>[7x]TNTLPHVAFYISVNRAISDEECTFNNSWLWKNEKGSRPFCKDANISLIYRVNLERSLQYGIVGSAAPDAKIVRISLDDDSTGAGIHLNDQLGYRQFGAS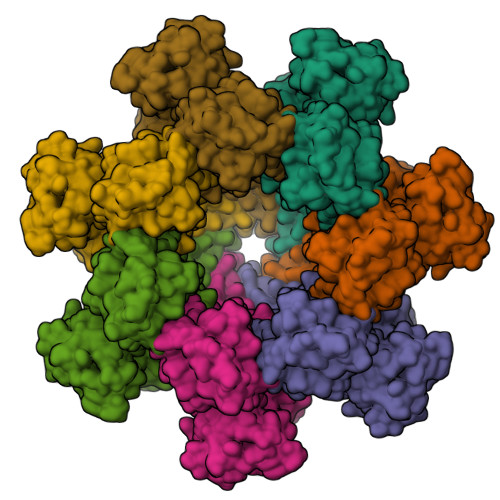YTTLDAYFREWSTDAIAQDYRFVFNASNNKAQILKTFPVDNINEKFERKEVSGFALGVTGGVEVSGDGPKAKLEARASYTQSRWLTYNTQDYRIERNAKNAQAVSFTWNRQQYATAESLLNRSTDALWVNTYPVDVNRISPLSYASFVPKMDVIYKASATETGSTDFIIDSSVNIRPIYNGAYKHYYVVGAHQFYHGFEDTPRRRITKSASFTVDWDHPVFTGGRPVNLQLASFNNRCIQVDAQGRLAANTCDSQQSAQSFIYDQLGRYVSASNTKLCLDGEALDALQPCNQNLTQRWEWRKGTDELTNVYSGESLGHDKQTGELGLYASSNDAVSLRTITAYTDVFNAQESSPILGYTQGKMNQQRVGQDHRLYVRAGAAIDALGSASDLLVGGNGGSLSSVDLSGVKSITATSGDFQYGGQQLVALTFTYQDGRQQTVGSKAYVTNAHEDRFDLPAAAKITQLKIWSDDWLVKGVQFDLN> MSAANADFELFRVFLEKTCGIVLGSNKQYLVSSRLNKLMEQQGIKSLGELVQRIQTQRGGLREMVVDAMTTNETLWFRDTYPFEVLKQRVLPELIKANGGQRLRIWSAACSSGQEPYSLSMAIDEFEKTNLGQLKAGVQIVATDLSGSMLTAAKAGEYDTLAMGRGLSPERLQR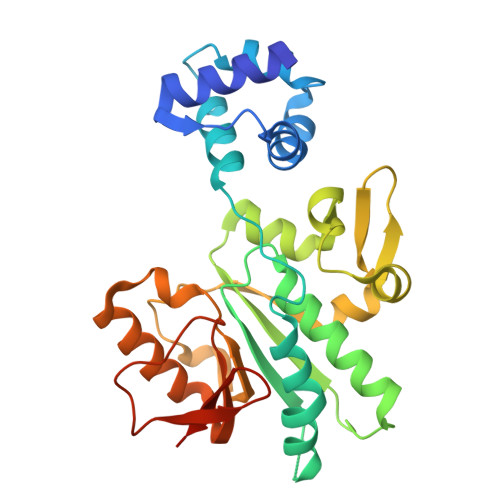YFDAKGPGRWAVKPAIRSRVEFRALNLLDSYASLGKFDMVFCRNVLIYFSAEVKRDILLRIHGTLKPGGYLFLGASEALNNLPDHYQMVQCSPGIIYRAKLEHHHHH>GAMSCVYAFGSNGQRQLGLGHDEDMDTPQRSVPGDDGAIVRKIACGGNHSVMLTNDGNLVGCGDNRRGELDSAQALRQVHDWRPVEVPAPVVDVACGWDTTVIVDADGRVWQRGGGCYEFTQQHVPLNSNDERIAVYGCFQNFV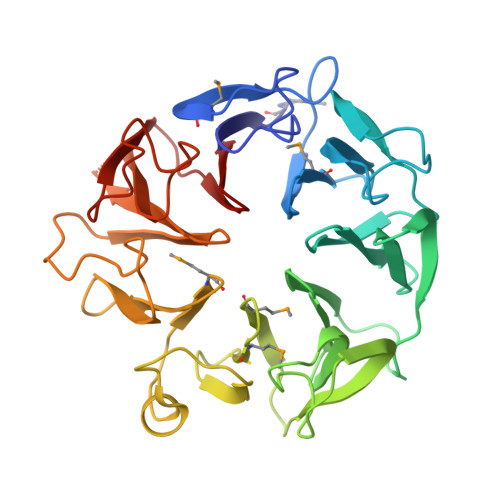VVQGTRVYGWGSNTKCQLQEPKSRSLKEPVLVYDTGSVAVDYVAMGKDFMVIVDEGGRIVHASGRLPTGFELKQQQKRHNLVVLCMWTSIHLWNARLNTVESFGRGTHSQLFPQERLDFPIVGVATGSEHGILTTANQEGKSHCYNVYCWGWGEHGNCGPQKGSQPGLQLVGQYSGKPRVFGGCATTWIVL[2x]> SVG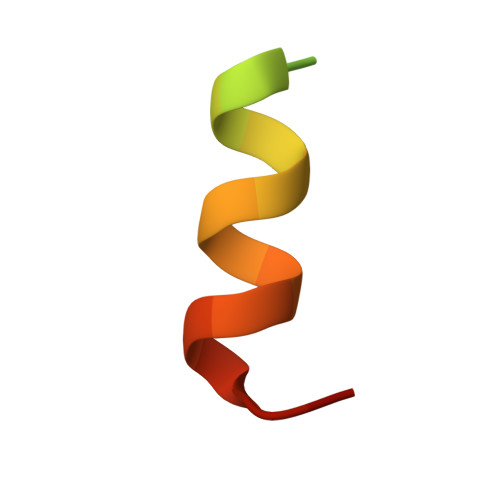TSVASAEQDELSQRLARLRDQV> MLKQVEIFTDGSCLGNPGPGGYGAILRYRGREKTFSAGYTRTTNNRMELMAAIVALEALKEHCEVILSTDSQYVRQGITQWIHNWKKRGWKTADGKPVKNVDLWQRLDAAL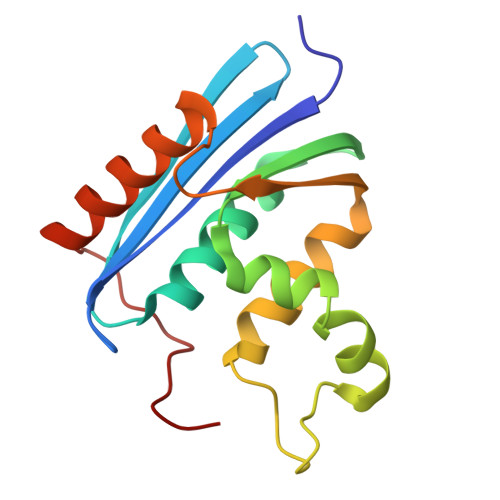GQHQIKWEWVKGHAGHPENERCDELARAAAMNPTLEDTGYQVEV> MSDLVLGLDIGIGSVGVGILNKVTGEIIHKNSRIFPAAQAENNLVRRTNRQGRRLTRRKKHRRVRLNRLFEESGLITDFTKISINLNPYQLRVKGLTDELSNEELFIALKNMVKHRGISYLDDASDDGNSSIGDYAQIVKENSKQLETKTPGQIQLERYQTYGQLRGDFTVEKDGKKHRLINVFPTSAYRSEALRILQTQQEFNPQITDEFINRYLEILTGKRKYYHGPGNEKSRTDYGRYRTSGETLDNIFGILIGKCTFYPDEFRAAKASYTAQEFNLLNDLNNLTVPTETKKLSKEQKNQIINYVKNEKAMGPAKLFKYIAKLLSCDVADIKGYRIDKSGKAEIHTFEAYRKMKTLETLDIEQMDRETLDKLAYVLTLNTEREGIQEALEHEFADGSFSQKQVDELVQFRKANSSIFGKGWHNFSVKLMMELIPELYETSEEQMTILTRLGKQKTTSSSNKTKYIDEKLLTEEIYNPVVAKSVRQAIKIVNAAIKEYGDFDNIVIEMARETNEDDEKKAIQKIQKANKDEKDAAMLKAANQYNGKAELPHSVFHGHKQLATKIRLWHQQGERCLYTGKTISIHDLINNSNQFEVDHILPLSITFDDSLANKVLVYATANQEKGQRTPYQALDSMDDAWSFRELKAFVRESKTLSNKKKEYLLTEEDISKFDVRKKFIERNLVDTRYASRVVLNALQEHFRAHKIDTKVSVVRGQFTSQLRRHWGIEKTRDTYHHHAVDALIIAASSQLNLWKKQKNTLVSYSEDQLLDIETGELISDDEYKESVFKAPYQHFVDTLKSKEFEDSILFSYQVDSKFNRKISDATIYATRQAKVGKDKADETYVLGKI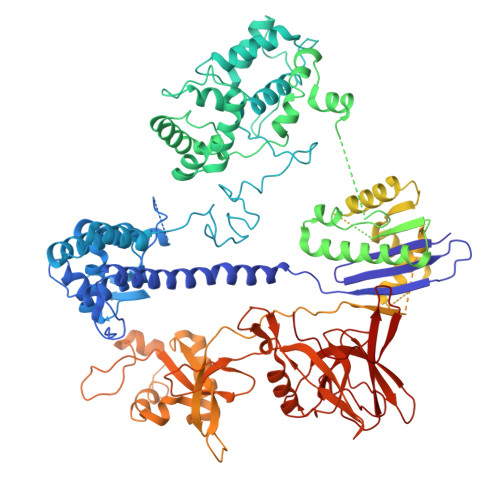KDIYTQDGYDAFMKIYKKDKSKFLMYRHDPQTFEKVIEPILENYPNKQINEKGKEVPCNPFLKYKEEHGYIRKYSKKGNGPEIKSLKYYDSKLGNHIDITPKDSNNKVVLQSVSPWRADVYFNKTTGKYEILGLKYADLQFEKGTGTYKISQEKYNDIKKKEGVDSDSEFKFTLYKNDLLLVKDTETKEQQLFRFLSRTMPKQKHYVELKPYDKQKFEGGEALIKVLGNVANSGQCKKGLGKSNISIYKVRTDVLGNQHIIKNEGDKPKLDF>[2x]SHGMAVTKVTVDGIEFPPTITPPGSSKSLTLLGAGVRGIEIEAIQIKVTAIGVYAEP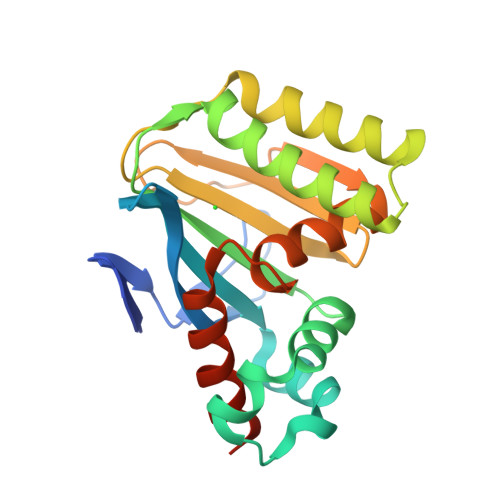EVIASHLQKWKGKSASELVEDDGFFKDLVQAPVEKLVKITMIKPLTGSQYGGAVEENIRDRLKALDKYSEAEEEALEEFREFFKTKSFPKGSVIFFHWSSPSTLQISVSTDGSLPEEAEATIENANVAAALLDVFLGKNSVSPSTKASVAEGISALLMKNKDEKEV>GSHGMYIIIAGIGRVGYTLAKSLSEKGHDIVLIDIDKDICKKASAEIDALVINGDCTKIKTLEDAGIEDADMYIAVTGKEEVNLMSSLLAKSYGINKTIARISEIEYKDVFERLGVDVVVSPELIAANYIEKLIERPG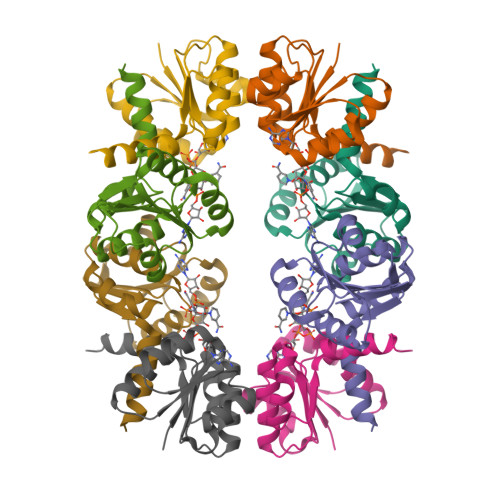IL[4x]> MGKGDPKKPRGKMSSYAFFVQTCREEHKKKHPDASVNFSEFSKKCSERWKTMSAKEKGKFEDMAKADKARYEREMKTYIPPKGETKKKFKDPNAPKRPPSAFFLFCSEYRPKIKGEHPGLSIGDVAKKLGEMWNN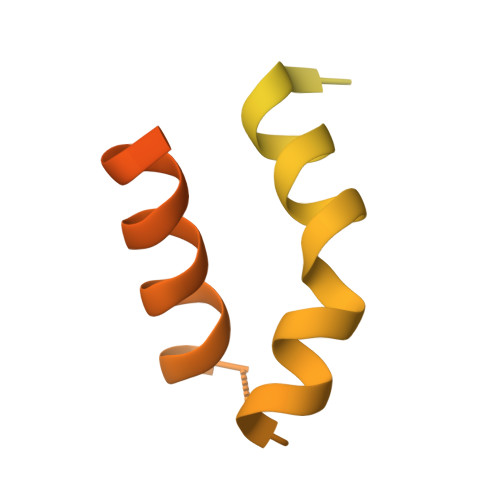TAADDKQPYEKKAAKLKEKYEKDIAAYR In this article we describe the crystal structure of TarS, an enzyme responsible for the glycosylation of wall teichoic acid polymers of the S. aureus cell wall, a process that has been shown to be specifically responsible for methicillin resistance in MRSA. TarS possesses a catalytic domain with a canonical GTA fold (one of two distinct A/B folds characteristic of nucleotide-sugar dependent glycosyltransferases) consisting of two closely associated α/β/α sandwich Rossmann motifs that abut and form a continuous central β-sheet. TarS possesses a D(91)XDD motif with aspartates coordinating a metal cation, a feature that is typical of the GTA superfamily. Altogether, TarS features a novel architecture with closely-associated trimerization domains connected by a linker region to three protruding catalytic domains that face away from each other.

Limited (thermolysin) proteolysis of the purified full-length TarS protein resulted in crystals diffracting to ~ 2.3 Å resolution, with SAD phasing using an iodide derivative revealing cleavage of the N-terminal region of the catalytic domain (1–216) and the structure of the TarS217-573 as described. TarS1-349, described above, was isolated by designing a structure-guided truncation mutant (based on the TarS217-573 structure) that resulted in a structure at 2.3 Å resolution with intact UDP-GlcNAc bound in the active site. The intact (rather than hydrolyzed) UDP-GlcNAc in the active site was achieved by soaking crystals in increased concentrations of substrate (50 mM) before freezing. Brief soaking of the TarS1-349 crystals with UDP-GlcNAc resulted in an enzyme-donor complex with UDP-GlcNAc trapped in the active site as evidenced by the ligand mFo-dFc simulated annealing omit electron density. Our analysis of the enzymatic mechanism of TarS was facilitated by the capture of various TarS1-349 structures encapsulating the catalytic domain in complex with metal and substrates. These include the native structure with bound Mn2+ (free enzyme), the UDP-GlcNAc bound structure in the presence and absence of Mn2+ (the binary Michaelis complex), and the UDP bound structure with Mn2+ (product complex). The first loop, designated as the catalytic site (CS) loop, contains the putative base catalyst D178 and moves towards the catalytic center in the presence of the intact UDP-GlcNAc donor substrate. The second loop, designated as the substrate access (SA) loop, is ordered only in the presence of UDP-GlcNAc and sterically occludes an otherwise open channel leading into the active site in the absence of the intact donor. Structural analysis revealed that Mn2+ is coordinated in a hexahedral manner, via a bivalent interaction with both side chain carboxylate oxygens of D93, the UDP-GlcNAc/UDP diphosphates O1A and O1B, as well as two ordered water molecules.

>MKFSVIVPTYNSEKYITELLNSLAKQDFPKTEFEVVVVDDCSTDQTLQIVEKYRNKLNLKVSQLETNSGGPGKPRNVALKQAEGEFVLFVDSDDYINKETLKDAAAFIDEHHSDVLLIKMKGVNGRGVPQSMFKETAPEVTLLNSRIIYTLSPTKIYRTALLKDNDIYFPEELKSAEDQLFTMKAYLNANRISVLSDKAYYYATKREGEHMSSAYVSPEDFYEVMRLIAVEILNADLEEAHKDQILAEFLNRHFSFSRTNGFSLKVKLEEQPQWINALGDFIQAVPERVDALVMSKLRPLLHYARAKDIDNYRTVEESYRQGQYYRFDIVDGKLNIQFNEGEPYFEGIDKLVPRGSAAAALEHHHHHH[2x]>SNASPDEQLLKQVSELLQQGEHAQALNVIQTLSDELQSRGDVKLAKADCLLETKQFELAQELLATIPLEYQDNSYKSLIAKLELHQQAAESPELKRLEQELAANPDNFELACELAVQYNQVGRDEEALEL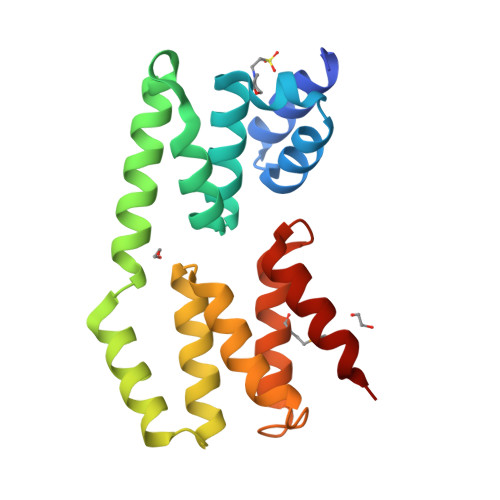LWNILKVNLGAQDGEVKKTFMDILSALGQGNAIASKYRRQLYSILY[2x]>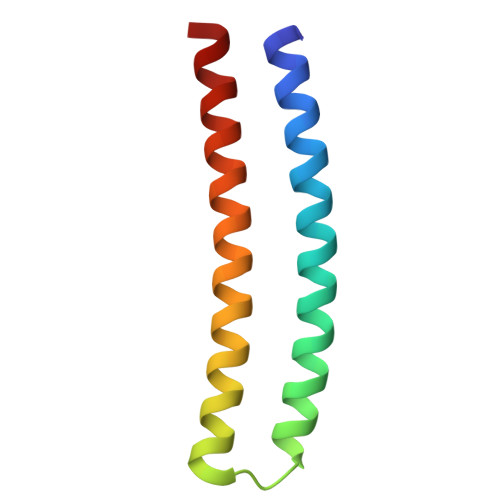 SSPVDEIDKEVKKLEEEAKKSQEEVERLKQEVEKASKAGLDHEGDSRIFKKIHDVVTKQIKVIIRLIEVYVRLVEIIL> MSKLEAILSQEVE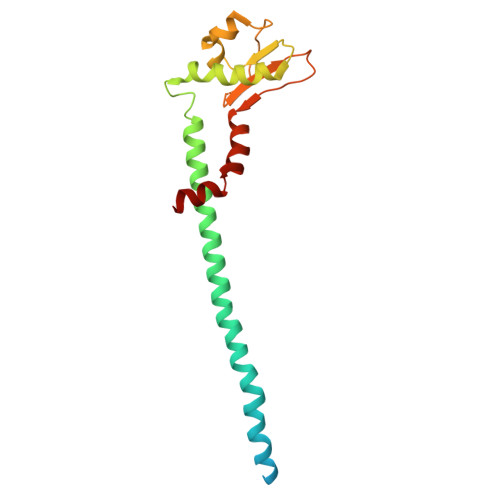AEIQALLQEAEAKAEAVKREAEEKAKALLQARERALEAQYRAALRRAESAGELLVATARTQARGEVLEEVRRRVREALEALPQKPEWPEVVRKLALEALEALPGAKALVANPEDLPHLEAMARERGVELQAEPALRLGVRAVGAEGKTQVENSLLARMDRAWDAMSSKVAQALWG Primary hyperoxaluria type I (PH1) is an autosomal recessive inborn error of metabolism caused by mutations in the AGXT gene, coding for the enzyme alanine-glyoxylate aminotransferase (AGT). AGT catalyzes the transamination of L-alanine to pyruvate and glyoxylate to glycine in the presence of pyridoxal 5′-phosphate (PLP) as cofactor. AGT homodimer has each protomer folded into a large N-terminal domain, a smaller C-terminal domain and a 22 amino acid long unstructured N-terminal tail that grabs the other subunit within the dimer. AGXT has two polymorphic variants, the most frequent (“wild-type”; AGT WT) called the major allele (haplotype) and a less common polymorphic variant called the minor allele (referred to as AGT LM) which appears in 20% of control subjects and 46% of PH1 patients.

The crystal structure of p.I340M has been determined at an unprecedented 1.9 Å resolution to improve our modeling efforts on PH1 causing mutants. The minor allele shows two single amino acid substitutions (p.P11L and p.I340M) among other genomic changes. The P11L and I340M polymorphisms are found in the dimer interface. P11L is expected to produce steric clashes with residues from the other subunit, which would explain the reduced stability and foldability of p.P11L, while I340M establishes several new favorable interactions hence explaining the stabilization observed for p.I340M, and the partial compensation of P11L destabilizing effect when they both occur in cis (i.e. the minor allele). Regarding the polymorphic variants, p.P11L and LM are kinetically destabilizing, while p.I340M enhances AGT kinetic stability compared to the WT protein, either in the apo- or the holo-form. The mutations analyzed on the minor allele occur in locations far from the dimerization interface, and with the exception of H83R, none of them are found near the active site. Modeling of Arg83 predicts a loss of interactions with PLP and the appearance of repulsions with surrounding residues, likely affecting the orientation of PLP (and/or PMP), which could explain the low catalytic activity, altered PLP/PMP binding mode and low stability as holo-protein of H83R. A295T, P319L and A368T substitutions are found in the vicinity of the domain:domain interface of AGT monomer, and cause an increase in the size of the side chain. Interestingly, these three mutations show more pronounced apo-AGT destabilization and deleterious effects in CHO cells (as total and soluble AGT protein levels) as closer the substitution is to the domain interface (P319L>A295T≥A368T), suggesting that a fine tuning of interactions in AGT domain:domain interface may be important for apo AGT kinetic stability and intracellular stability and foldability.

>[2x]MASHKLLVTPPKALLKPLSIPNQLLLGPGPSNLPPRIMAAGGLQMIGSMSKDMYQIMDEIKEGIQYVFQTRNPLTLVISGSGHCALEAALVNVLEPGDSFLVGANGIWGQRAVDIGERIGARVHPMTKDPGGHYTLQEVEEGLAQHKPVLLFLTHGESSTGVLQPLDGFGELCHRYKCLLLVDSVASLGGTPLYMDRQGIDILYSGSQKALNAPPGTSLISFSDKAKKKMYSRKTKPFSFYLDIKWLANFWGCDDQPRMYHHTIPVISLYSLRESLALIAEQGLENSWRQHREAAAYLHGRLQALGLQLFVKDPALRLPTVTTVAVPAGYDWRDIVSYVMDHFDIEIMGGLGPSTGKVLRIGLLGCNATRENVDRVTEALRAALVAQA Lipocalins are a superfamily of functionally diverse proteins with remarkably conserved tertiary structure despite significant sequence variation. These ~ 20 kDa proteins form an eight-stranded antiparallel β-barrel enclosing an internal ligand-binding pocket. The precise biological function of some lipocalin family proteins is not yet clear, even for those discovered more than two decades ago. This includes the first bacterial lipocalin protein identified, Escherichia coli lipocalin Blc. Blc is a membrane-associated protein anchored to the outer membrane by a covalently bound N-terminal cysteine lipid, and it faces the periplasmic space.

However, we were able to determine the structure of wtBlc-split protein at 1.94 Å resolution. The wtBlc-split asymmetric unit cell contained three ‘split’ molecules that differ primarily in the area of the two β-strands adjacent to the split point. Two fragments of the split protein together fully reconstitute the typical lipocalin fold. During structure refinement, we discovered a well-defined positive difference density map area in the binding pocket of one of the three ‘split’ molecules in the asymmetric unit. Based on the shape of the density as well as previous observations including color of the protein, absorbance, and fluorescence spectra, we suggested the presence of the heme B molecule in the structure. The heme molecule occupied the same hydrophobic cavity of the lipocalin as it was previously showed for vaccenic acid. In the binding pocket formed by chains E and F of the structure, there are 19 amino acid residues containing atoms within a 4.0 Å distance from the ligand (Glu45, Phe53, Glu54, Leu57, Val60, Asn76, Lys77, Gly78, Ser89, Phe108, Tyr113, Gly114, Gly115, Tyr116, Val130, Pro133, Tyr137, Trp139, and Leu141). Phe53 and Trp139 form π-stacking interactions with the porphyrin rings IV and II. The side-chain hydroxyl of Tyr137 and backbone amide of Gly113 stabilize one of the propionate groups of heme by hydrogen bonds. There are two additional amino acid residues from the adjacent ‘split’ molecule in the asymmetric unit (Ser148 and Glu150 from chain D) that contribute interactions with heme at the solvent front.

>[3x]MGHHHHHHLESTSLYKKSSSTPPRGVTVVNNFDAKRYLGTWYEIARFDHRFERGLEKVTATYSLRDDGGLNVINKGYNPDRGMWQQSEGKAYFTGAPTRAALKVSFF;>[3x]MGPFYGGYNVIALDREYRHALVCGPDRDYLWILSRTPTISDEVKQEMLAVATREGFDVSKFIWVQQPGS>LTEELRTFPINAQGDTAVLSLKEIKKGQQVFNAACAQCHALGVTRTNPDVNLSPEALALATPPRDNIAALVDYIKNPT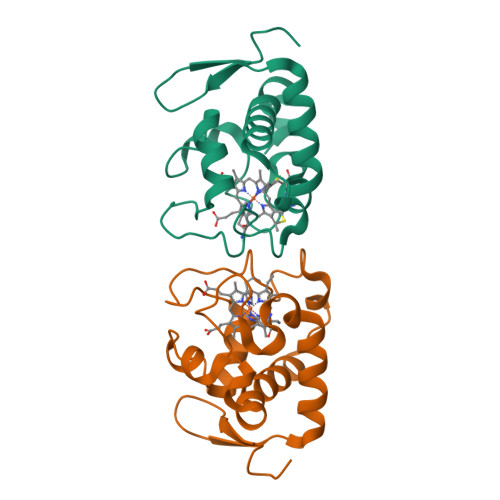TYDGFVEISELHPSLKSSDIFPKMRNISEDDLYNVAGYILLQPKVRGEQWG[2x]>[2x]SGVDLGTENLYFQSMANLRKVLISDSLDPCCRKILQDGGLQVVEKQNLSKEELIAELQDCEGLIVRSATKVTADVINAAEKLQVVGRAGTGVDNVDLEAA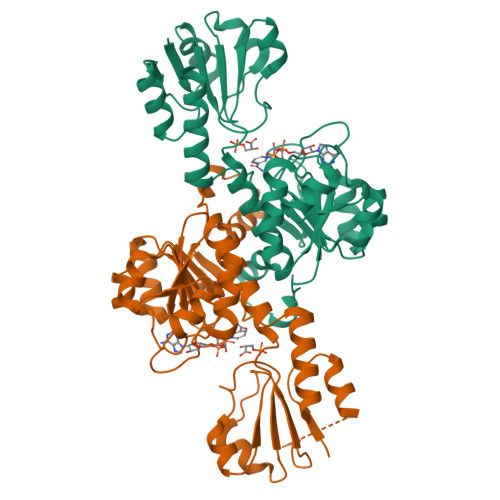TRKGILVMNTPNGNSLSAAELTCGMIMCLARQIPQATASMKDGKWERKKFMGTELNGKTLGILGLGRIGREVATRMQSFGMKTIGYDPIISPEVSASFGVQQLPLEEIWPLCDFITVHTPLLPSTTGLLNDNTFAQCKKGVRVVNCARGGIVDEGALLRALQSGQCAGAALDVFTEEPPRDRALVDHENVISCPHLGASTKEAQSRCGEEIAVQFVDMVKGKSLTGV> MTIGQKNTNIDPRFPHH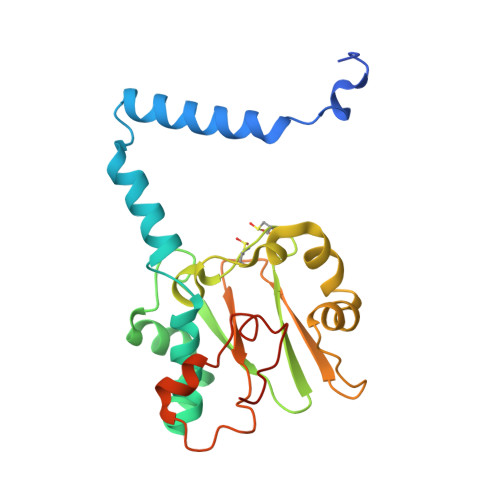HPRPQSFWEARAKALESLLIEKGHLSSDAIERVIKHYEHELGPMNGAKVVAKAWTDPAFKQRLLEDSETVLRELGYYGLQGEHIRVVENTDTVHNVVVCTLCSCYPWPLLGLPPSWYKEPAYRARVVKEPRQVLKEFGLDLPDSVEIRVWDSSSEIRFMVLPQRPEGTEGMTEEELAKLVTRDSMIGVAKIEPPKVTVG> SMQGPRTRARLGANEVLLVVGGFGSQQSPIDVVEKYDPKTQEWSFLPSITRKRRYVASVSLHDRIYVIGGYDGRSRLSSVECLDYTADEDGVWYSVAPMNVRRGLAGATTLGDMIYVSGGFDGSRRHTSMERYDPNIDQWSMLGDMQTAREGAGLVVASGVIYCLGGYDGLNILNSVEKYDPH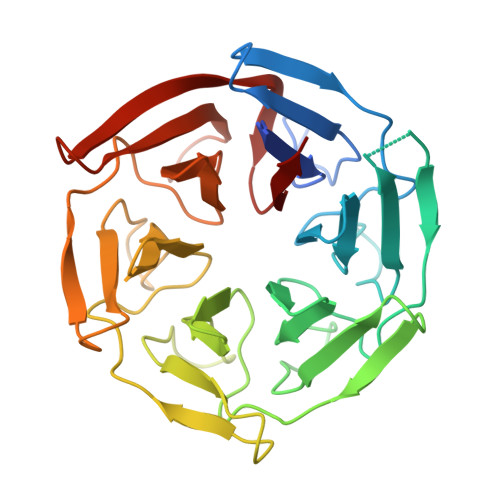TGHWTNVTPMATKRSGAGVALLNDHIYVVGGFDGTAHLSSVEAYNIRTDSWTTVTSMTTPRCYVGATVLRGRLYAIAGYDGNSLLSSIECYDPIIDSWEVVTSMGTQRCDAGVCVLRE>MKVTFEQLKAAFNRVLISRGVDSETADACAEMFARTTESGVYSHGVNRFPRFIQQLENGDIIPDAQPKRITSLGAIEQWDAQRSIGNLTAKKMMDRAIELAADHGIGLVALRNANHWMRGGSYGWQAAEKGYIGICWTNSIAVMPPWGAKECRIGTNPLIVAIPSTPITMVDMSMSMFSYGMLEVNRLAGRQLPVDGGFDDEGNLTKEPGVIEKNRRILPMGYWKGSGMSIVLDMIATLLSDGASVAEVTQDNSDEYGISQIFIA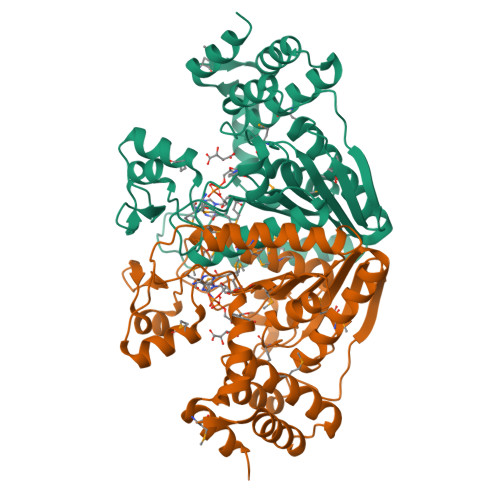IEVDKLIDGPTRDAKLQRIMDYVTSAERADENQAIRLPGHEFTTLLAENRRNGITVDDSVWAKIQALLEHHHHHH[8x]> MGSSHHHHHHGSMNHYTRWLELKEQNPGKYARDIAGLMNIREAELAFARVTHDAWRMHGDIRDILAALESVGETKCICRNEYAVHEQVGTFTNQHLNGHAGLILNPRALDLRLFLNQWASVFHIKENTARGERQSIQFFDHQGDALLKVYATDNTDMAAWSELLARFITDENTPLELKAVDAPVVQTRADATVVEQEWRAMTDVHQFFTLLKRHNLTRQQAFNLVADDLA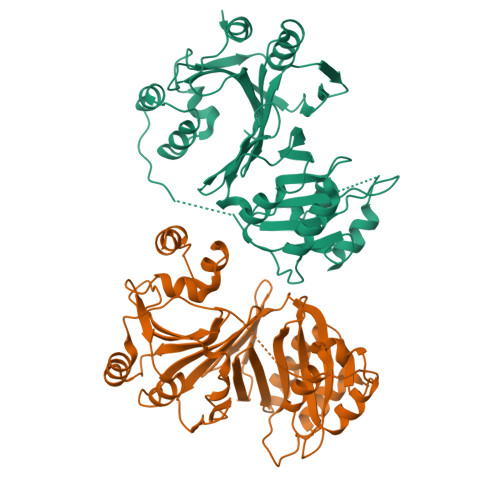CKVSNSALAQILESAQQDGNEIMVFVGNRGCVQIFTGVVEKVVPMKGWLNIFNPTFTLHLLEESIAEAWVTRKPTSDGYVTSLELFAHDGTQIAQLYGQRTEGDQEQAQWRKQIASLIPEGVAA> MHETKQGGEKRFTGAICRCSHRYNSMEVKMAATTIGGAAAAEAPLLDKKWLTFALAIYTVFYLWVRWYEGVYGWSAGLDSFAPEFETYWMNFLYTEIVLEIVTASILWGYLWKTRDRNLAALTPREELRRNFTHLVWLVAYAWAIYWGASYFTEQDGTWHQTIVRDTDFTPSHIIEFYLSYPIYIITGFAAFIYAKTRLPFFAKGISLPYLVLVVGPFMILPNVGLNEWGHTFWFMEELFVAPLHYGFVIFGWLALAVM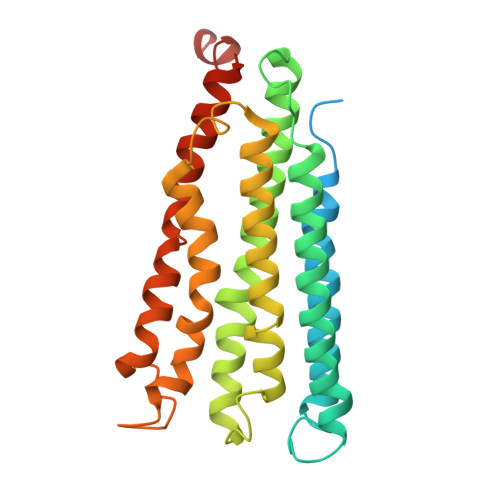GTLTQTFYSFAQGGLGQSLCEAVDEGLIAK> EA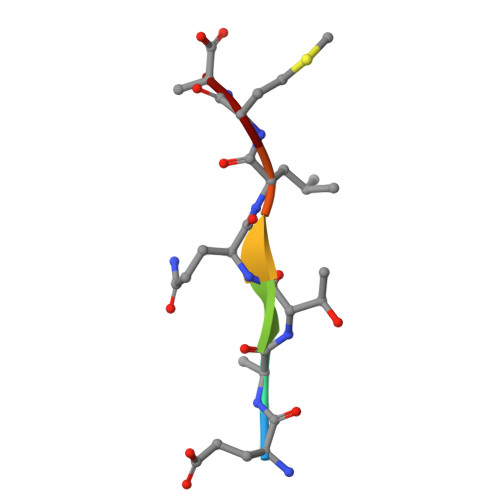TQLMN>[2x]SEDCENIFHDNAYLLKLDCEAGRVDPVEFDDISDEEIYEITVDVGVSSEDQEKVAKIIRECIAQVSTQDCTKFSEIYDCYMKKKICNYYPENMGSGHHHHHHHH;>[2x]KCPQPKTLDEFTIIQNLQPQYQFRDYFIATCKQGYQLIEGNQVLHSFTAVCQDDGTWHRAMPRCKIKDCGQPRNLPNGDFRYTTTMGVNTYKARIQYYCHEPYYKMQTRAGSRESEQGVYTCTAQGIWKNEQKGEKIPRCLPVCGKPVNPVEQRQRIIGGQKAKMGNFPWQVFTNIHGRGGGALLGDRWILTAAHTLYPKEHEAQSNASLDVFLGHTNVEELMKLGNHPIRRVSVHPDYRQDESYNFEGDIALLELENSVTLGPNLLPICLPDNDTFYDLGLMGYVSGFGVMEEKIAHDLRF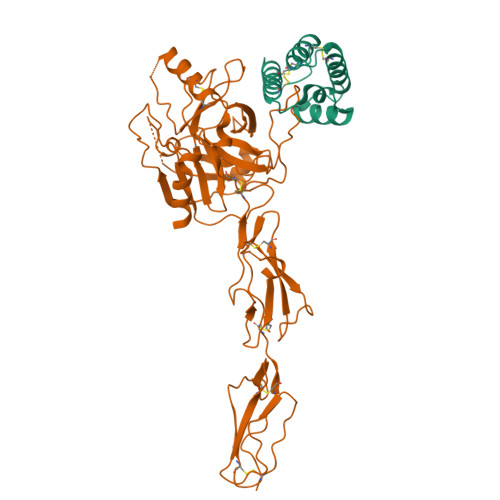VRLPVANPQACENWLRGKNRMDVFSQNMFCAGHPSLKQDACQGDAGGVFAVRDPNTDRWVATGIVSWGIGCSRGYGFYTKVLNYVDWIKKEMEEEDGSGHHHHHHHH>[4x]TKPFTLPILTISELTNSRFPIPIEQLYTAPNENNVVQCQNGRCTLDGELQGTTQLLSSAVCSYRGRTVANSGDYWDQNLLQLTYPSGASYDPTDEVPAPLGTQDFSGILYGVLTQDNVSEGTGEAKNAKGVYISTTSGKFTPKIGSIGLHSITENVHPNQQSRFTPVGVAQNENTPFQQWVLPHYAGALALNTNLAPAVAPTFPGEQLLFFRSRVPCVQGLRGQDAFIDCLLPQEWVNHFYQEAAPSQADVALIRYVNPDTGRTLFEAKLHRSGFITVSHTGAYPLVVPPNGHFRFDSWVNQFYSLAPM

Human noroviruses (huNoVs), members of the Norovirus genus of the Caliciviridae family, are the leading cause of acute gastroenteritis (AGE) and are associated with almost 20% of all AGE cases worldwide. The major capsid protein (VP1) is composed of a shell (S) domain and a protruding (P) domain, and the P domain is further divided into the P1 and P2 subdomains. The P2 subdomain is the main determinant of NoV diversity, antigenicity, and glycan binding patterns. In conclusion, GII.13/21 huNoVs have developed a novel GBS that interacts with glycans via the common β-Gal through a unique glycan binding mode.

OIF P domain was reported to bind Lea antigen but the GII. P domains in our study did not, three reverse mutants of the GII.13 (SC1065/2016) P domain were constructed to explore the role of these amino acids in glycan binding. These included a single mutation (N297Y or G361E) and a double mutation (N297Y/G361E), aiming to restore the Lea binding function. Unexpectedly, oligosaccharide-based binding assays showed that all mutant P domains retained their original pattern of binding to Lec/lac/mucin core 2 glycans and did not bind to Lea antigen. Also, the single mutant N297Y and the double mutant N297Y/G361E showed stronger binding signals to all Lec/Lac/mucin core 2 glycans and particularly to mucin core 2, while E361 showed the same binding affinity for the glycans as the native P proteins. We determined the crystal structure of the SC1065/2016 N297Y mutant. Y297 in the crystal structure of an SC1065 N297Y mutant displayed an orientation opposite that in GII. Also, an attempt to shift the binding of GII. SC1065/2016 to Lea by reverse mutation of residues 297 and/or 361 failed.> MGSSHHHHHHMKNARRVSLSPLILRSLAELQDGLNTVVDKNWRQLRRPGDWSLAITMEAAELLDSYPWKWWKNVKAQPDLQNVKIELTDILHFSLSGAMQVSDENSGAVHKAEAGSNGESGKHWCYFDQPRALPAAGGAEYVACVETPGSSLSAPVSADECDLADFMFFPLSDTNNALASFQNIIRLASLQRFQLVTSAVIAAADDIGFNLVAYYVAKHTLNGIRQMKGYKDGTYVKVQKGVEDNELLHGCISPFSL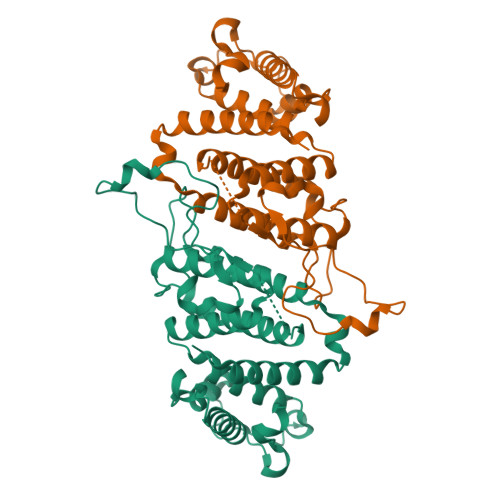DDVTNEGNYKTKWDDIMHRVYDAFGTPKEERLNIGHWLKS> MGPSLDF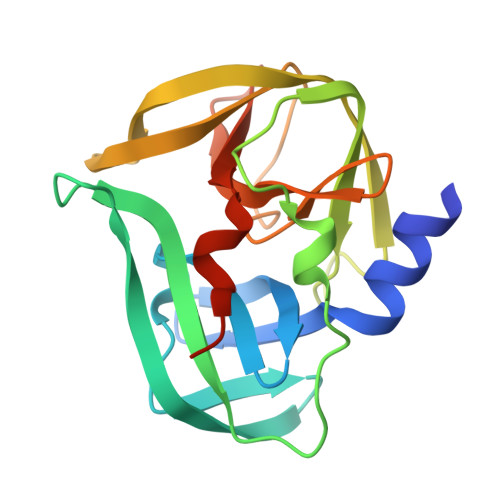ALSLLRRNIRQVQTDQGHFTMLGVRDRLAVLPRHSQPGKTIWIEHKLVNVLDAVELVDEQGVNLELTLITLDTNEKFRDITKFIPENISTASDATLVINTEHMPSMFVPVGDVVQYGFLNLSGKPTHRTMMYNFPTKAGQAGGVVTSVGKVIGIHIGGNGRQGFCAGLKRSYFASEQHHHHHH>KPGAPWWKSAVFYQVYPRSFKDTNGDGIGDFKGLTEKLDYLKGLGIDAIWINPHYASPNTDNGYDISDYREVMKEYGTMEDFDRLMAELKKRGMRLMVDVVINHSSDQHEWFKSSRASKDNPYRDYYFWRDGKDGHEPNNYPSFFGGSAWEKDPVTGQYYLHYFGRQQPDLNWDTPKLREELYAMLRFWLDKGVSGMRFDTVATYSKTPGFPDLTPEQMKNFAEAYTQGPNLHRYLQEMHEKVFDHYDAVTAGEIFGAPLNQVPLFIDSRRKELDMAFTFDLIRYDRALDRWHTIPRTLADFRQTIDKVDAIAGEYGWNTFFLGNHDNPRAVSHFGDDRPQWREASAKALATVT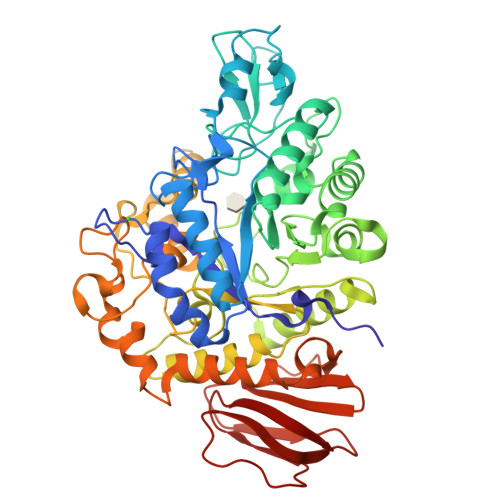LTQRGTPFIFQGDELGMTNYPFKTLQDFDDIEVKGFFQDYVETGKATAEELLTNVALTSRDNARTPFQWDDSANAGFTTGKPWLKVNPNYTEINAAREIGDPKSVYSFYRNLISIRHETPALSTGSYRDIDPSNADVYAYTRSQDGETYLVVVNFKAEPRSFTLPDGMHIAETLIESSSPAAPAAGAASLELQPWQSGIYKVK[2x]> DAAQPARRARRTYEAYPAKPKCPAVCTCTKDNALCENARSIPRTVPPDVISLSFVRSGFTEISEGSFLFTPSLQLLLFTSNSFDVISDDAFIGL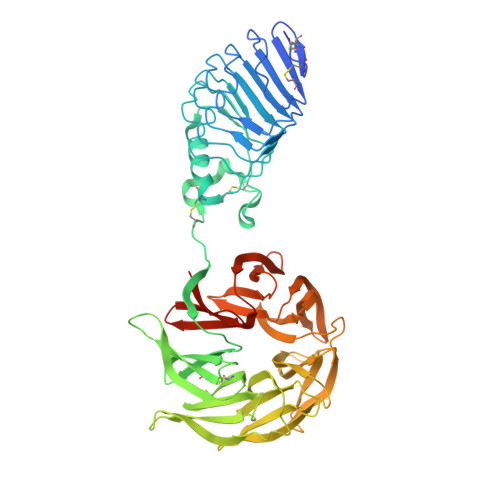PHLEYLFIENNNIKSISRHTFRGLKSLIHLSLANNNLQTLPKDIFKGLDSLTNVDLRGNSFNCDCKLKWLVEWLGHTNATVEDIYCEGPPEYKKRKINSLSSKDFDCIITEFAKSQDLPYQSLSIDTFSYLNDEYVVIAQPFTGKCIFLEWDHVEKTFRNYDNITGTSTVVCKPIVIETQLYVIVAQLFGGSHIYKRDSFANKFIKIQDIEILKIRKPNDIETFKIENNWYFVVADSSKAGFTTIYKWNGNGFYSHQSLHAWYRDTDVEYLEIVRTPQTLRTPHLILSSSSQRPVIYQWNKATQLFTNQTDIPNMEDVYAVKHFSVKGDVYICLTRFIGDSKVMKWGGSSFQDIQAMPSRGSMVFQPLQINNYQYAILGSDYSFTQVYNWDAEKAKFVKFQELNVQAPRSFTHVSINKRNFLFASSFKGNTQIYKHVIVDLSAKHHHHHH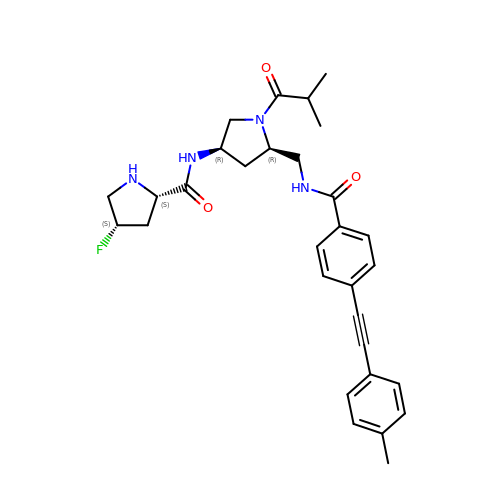(2S,4S)-4-fluoranyl-N-[(3R,5R)-5-[[[4-[2-(4-methylphenyl)ethynyl]phenyl]carbonylamino]methyl]-1-(2-methylpropanoyl)pyrrolidin-3-yl]pyrrolidine-2-carboxamide | C30 H35 F N4 O3 | JWAHLGPUOAMWDB-YAOOYPAMSA-N5-ACETYLAMINO-4-AMINO-6-(PHENETHYL-PROPYL-CARBAMOYL)-5,6-DIHYDRO-4H-PYRAN-2-CARBOXYLIC ACID | 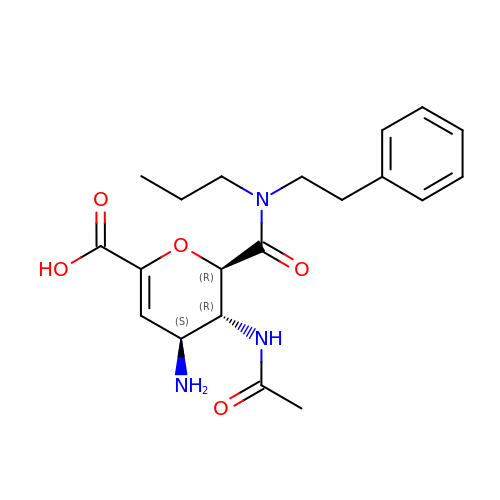C20 H27 N3 O5 | ZNRGSYNQOLEMKF-CGTJXYLNSA-N~{N}-(1~{H}-indazol-4-yl)methanesulfonamide | 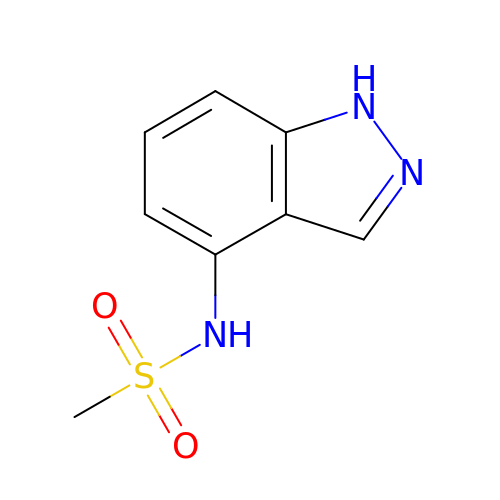C8 H9 N3 O2 S | CAMWAWBWBXRPRP-UHFFFAOYSA-N>GSSPVVKRLLGWKKSAGGSGGAGGGEQNGQ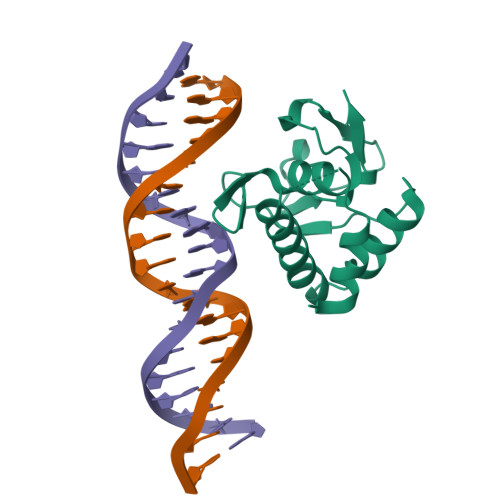EEKWSEKAVKSLVKKLKKTGRLDELEKAITTQNMNTKCVTIPRSLDGRLQVSHRKGLPHVIYCRLWRWPDLHSHHELKAIENCEYAFNLKKDEVCVNPYHYQRVETPSS[2x]>[2x]MASRKFFVGGNWKMNGTLESIKALVETLNSAQLDPNTEVVVAPPAIYLPFARSKLKKPKEIQV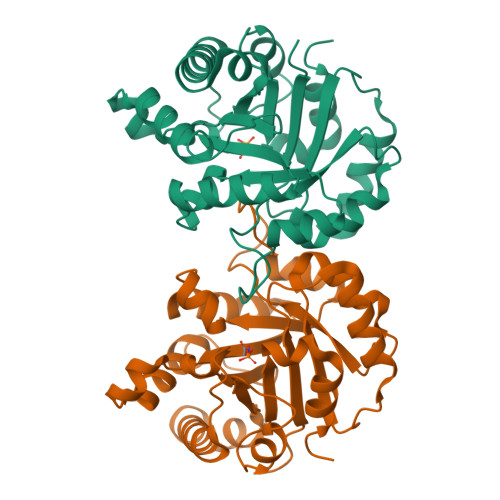AAQNCYTKPNGAFTGEISAEMLKDLGVPWVILGHSERRTIFGESDELIAEKVKYALDQGLKVIACIGETLEEREAGKTMEVVARQILKAIADKIKDWSNVVIAYEPVWAIGTGKVATPEQAQEVHAALRKWLKENVSPEVAESTRIIYGGSVNAANCKELAKQPDIDGFLVGGASLKAPEFVDIINARQ> ESQTTSRCHPHDLEALRDFIAHLEPKPDGWINSSSSTDCCNWTGITCNSNNTGRVIRLELG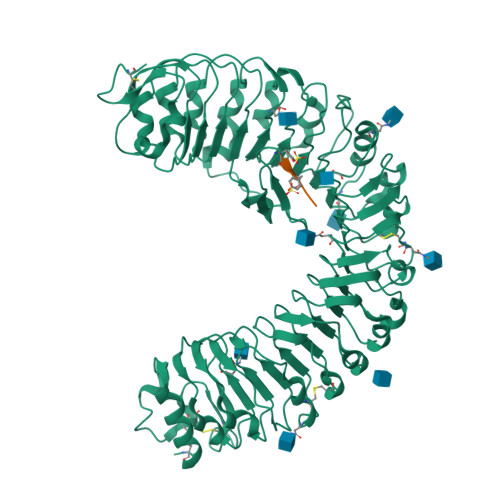NKKLSGKLSESLGKLDEIRVLNLSRNFIKDSIPLSIFNLKNLQTLDLSSNDLSGGIPTSINLPALQSFDLSSNKFNGSLPSHICHNSTQIRVVKLAVNYFAGNFTSGFGKCVLLEHLCLGMNDLTGNIPEDLFHLKRLNLLGIQENRLSGSLSREIRNLSSLVRLDVSWNLFSGEIPDVFDELPQLKFFLGQTNGFIGGIPKSLANSPSLNLLNLRNNSLSGRLMLNCTAMIALNSLDLGTNRFNGRLPENLPDCKRLKNVNLARNTFHGQVPESFKNFESLSYFSLSNSSLANISSALGILQHCKNLTTLVLTLNFHGEALPDDSSLHFEKLKVLVVANCRLTGSMPRWLSSSNELQLLDLSWNRLTGAIPSWIGDFKALFYLDLSNNSFTGEIPKSLTKLESLTSRNISVNEPSPDFPFFMKRNESARALQYNQIFGFPPTIELGHNNLSGPIWEEFGNLKKLHVFDLKWNALSGSIPSSLSGMTSLEALDLSNNRLSGSIPVSLQQLSFLSKFSVAYNNLSGVIPSGGQFQTFPNSSFESNHLCGEHRFPCSEGTESALIKHHHHHH;> YIYTQ> SNAMSFLTLKDVDLKDKKVLVRVDFNVPVKDGKVTSKVRIEAAIPTIQYILDQGGAVILMSHLGRPTEGEYDSQFSLEPVAKALSEIINKPVKFAKDWLDGVDVKAGEIVMCENVRFNSGEKKSTDDLSKKIASLGDVFVMDAFATAHRAQASTYGVAKYIP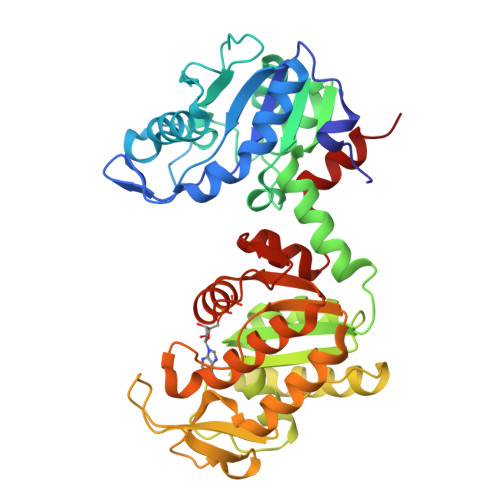VACAGILLTNEIQALEKALKSPKKPMAAIVGGSKVSTKLSVLNNLLDKVEILIVGGGIANTFIKAEGFDVGNSLYEQDLVAEATEILAKAKALGVNIPVPVDVRVAKEFSENAQAIIKKVSDVVADEMILDIGPESQKIIAELLKSANTILWNGPVGVFEFDNFAEGTKALSLAIAQSHAFSVAGGGDTIAAIEKFGIKDQVSYISTAGGAFLEFLEGKKLPAIEILKEKAIR2-{5-[AMINO(IMINIO)METHYL]-1H-BENZIMIDAZOL-2-YL}-6-BROMO-4-METHYLBENZENOLATE | C15 H13 Br N4 O | 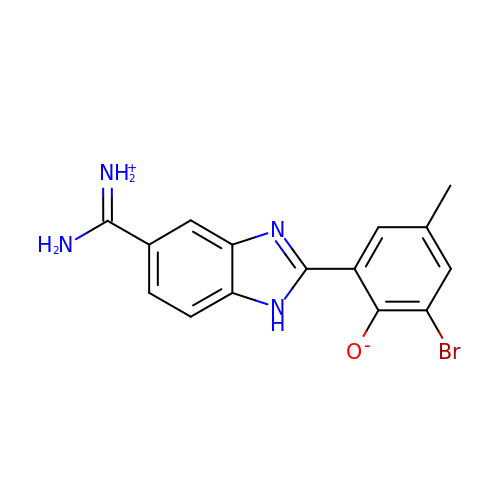XKCHOMIJYLHXLI-UHFFFAOYSA-N> MAHHHHHHVDDDDKMVHHDGFQT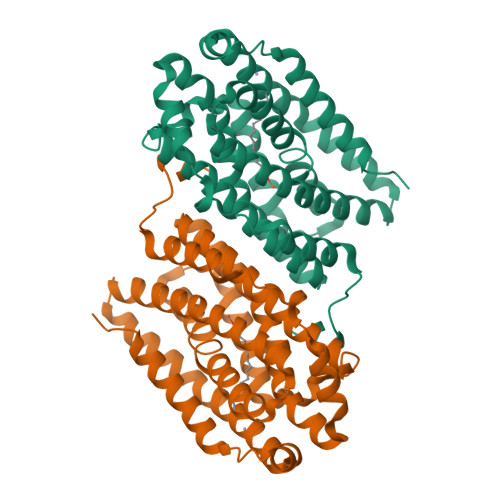VKATIDWEHPMFKLYEKAKRNGKWNPADIDFSQDQKDFASLTSEEKISALPLVAGFSAGEEAITLDILPMAHALARQGRLEDVLFLTTFMHDEAKHVEMFSRWQQAVGIGQMDLSVFHNDHYKRIFYEALPEAMNRLYADDSPEAVIRAATVYNMIVEGTLAESGYYTFRQIYKKAGLFPGLLQGIDYLNMDEGRHIQFGIYTIQRIVNEDERYYELFIRYMDELWPHVIGYVDYLTELGKRQQQLARTYALEIDYDLLRHYVIKQFNLRKKQISRTKRVDVVEGLEKTAAES>MGSIGSMGKPIEGFLVAAIQFPVPIVNSRKDIDHNIESIIRTLHATKAGYPGVELIIFPEYSTQGLNTAKWLSEEFLLDVPGKETELYAKACKEAKVYGVFSIMERNPDSNKNPYNTAIIID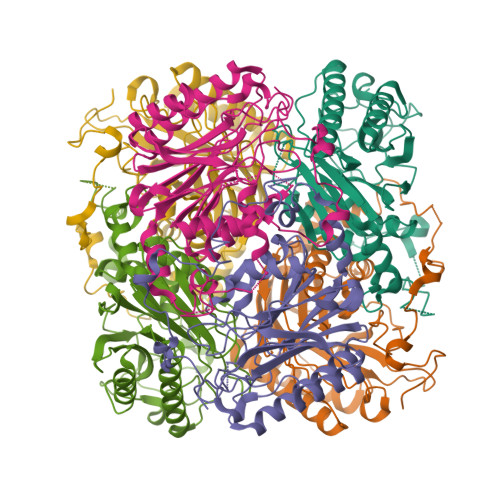PQGEIILKYRKLFPWNPIEPWYPGDLGMPVCEGPGGSKLAVCISHDGMIPELAREAAYKGCNVYIRISGYSTQVNDQWILTNRSNAWHNLMYTVSVNLAGYDNVFYYFGEGQICNFDGTTLVQGHRNPWEIVTGEIYPKMADNARLSWGLENNIYNLGHRGYVAKPGGEHDAGLTYIKDLAAGKYKLPWEDHMKIKDGSIYGYPTTGGRFGK[6x]>GIDPFTMTPSEDFVVTDRGGIVENSHRVHAAVVDAKGRLLYALGNPTRMTLARSAAKPAQALAILETEGVAGYGFDDADIALMCASHSSEDRHIARTRAMLSKIKAEEADLRCGGHPSLSEMVNRSWIKQDFIPTAVCSNCSGKHVGMLAGARAIGAGTDGYHLPDHPMQGRVKRTVAELCDLDAGDVEWGTDGCNLPTPAFPLDRLGRIYAKLASAADGSDAGEGQSTRCAALAHIFRAMARHPEMVAGEGRYCTMLMRAFDGALVGKLGADASYAIGVRASDATRQLGTDGALGISVKIEDGNLEMLYAVVTELLERLGIGSPDVRSQLASFHHPQRVNTMGVTTGGVSFPFKLRGSKSNVDDPRLAAVAR[2x]

Rhizobium etli, a nitrogen-fixing bacterial symbiont of legume plants, encodes an essential l-asparaginase (ReAV) with no sequence homology to known enzymes with this activity. High-resolution crystal structures of ReAV show indeed a structurally distinct, dimeric enzyme, with some resemblance to glutaminases and β-lactamases. The active site of ReAV, deduced from structural comparisons and confirmed by mutagenesis experiments, contains a highly specific Zn2+ binding site without a catalytic role. There are two Ser-Lys tandems, all connected through a network of H-bonds to the Zn center, and three tightly bound water molecules near Ser48, which clearly indicate the catalytic nucleophile.

All the crystal structures reveal the presence of a zinc ion in the active site area. The zinc ion was found near helix H9 and the loop connecting strands B5–B6, with a tetrahedral coordination sphere formed by Cys135, Lys138, Cys189 and a water molecule (w1). The distance between the water molecule w1 and Zn2+ is in the range ~1.89–2.05 Å and the position of this water is the same in all structures. The position of Cys189 is nearly identical in all the structures and is additionally held in place by an H-bond to the side chain of His139.>MLPKFDPTNQKACLSLLEDLTTNVKQIQDSVLEAILSRNAQTEYLRGFLNGQVDKQNFKKNVPVVTYEDIRSYIDRIANGEPSDLICDRPISVLLTSSGTSGGVPKLIPLTTEDLEQRISFSSLYAPLLYKHIDGLSEGKSLIFYFVTRESKTANGLMVRTMVTSFLKSIKQTNSFLWDSLQVSPHAITTCADTTQSMYCQLLCGLLERDNVARLGAPFASSFLKVIKFLEDH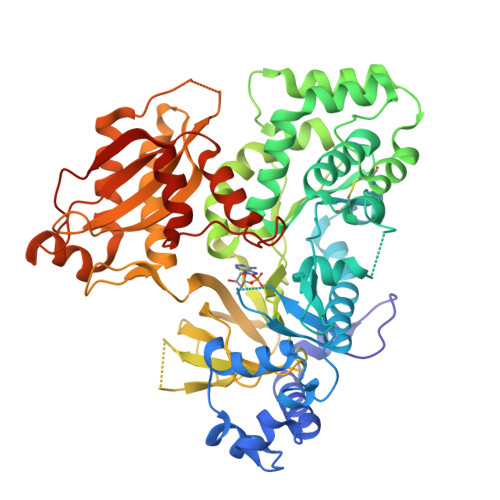WPELCSNIRTGRLSDWITDATCTSGIGKFLTAPNPELASLIEQECSKTSWEAILKRLWPKAKCIESIITGTMAQYIPLLEFYSGGLPLTSSFYGSSECFMGVNFNPLCKPSDVSYTIIPCMGYFEFLEVEKDHQEAGHDPTEKPVVVDLVDVKIGHDYEPVVTTFSGLYRYRVGDVLRATGFYNNAPHFCFVGRQKVVLSIDMDKTYEDDLLKAVTNAKLLLEPHDLMLMDFTSRVDSSSFPGHYVIYWELGSKVKDAKFEPNRDVMEECCFTVEESLDAVYRKGRKNDKNIGPLEIKVVKPGAFDELMNFFLSRGSSVSQYKTPRSVTNEEALKILEANVISEFLSRKIPSWELHELHSGR[4x]> PITVIVSGATGFIAQHVVKQLLAKNYQVIGTVRSTAKGDHLLKLFNNPKNLSYEIVEDVGTKGAFDKVLQKHGEAKVFLHLASPFHFNVTDVEKELLLPAVDGTKNVLQAIYNFGNNIEKVVITSSYAAISTASKEADKNAIITEKDWNEISWQDALLNPVNGYRGSKKFAEKAAWDFIKSNDNVKFSLSTINPSFVFGPQSFGSEIKQSLNTSSEIINSILKLKPNDSIPASKGGWVDVRDVAKAHIIAFENEDAKNQRILLNSGRFTSQSLVDIINDKFPDLKGKIPVDEPGSDKSVIAESLATIDDTKSRELLGFEYYNLEQSVYDTVEQIVNA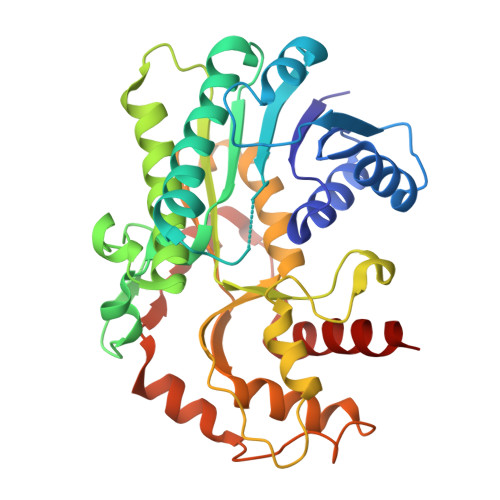HK>MLSEGTHLRPYETLGAHADTMDGVTGTRFSVWAPNARRVSVVGQFNYWDGRRHPMRLRKESGIWELFIPGAHNGQLYKYEMIDANGNLRLKSDPYAFEAQMRPETASLICGLPEKVVQTEERKKANQFDAPISIYEVHLGSWRRHTDNNFWLSYRELADQLVPYAKWMGFTHLELLPINEHPFDGSWGYQPTGLYAPTRRFGTRDDFRYFIDAAHAAGLNVILDWVPGHFPTDDFALAEFDGTNLYEHSDPREGYHQDWNTLIYNYGRREVSNFLVGNALYWIERFGIDALRVDAVASMIYRDYSRKEGEWIPNEFGGRENLEAIEFLRNTNRILGEQVSGAVTMAEESTDFPGVSRPQDMGGLGFWYKWNLGWMHDTLDYMKLDPVYRQYHHDKLTFGILYNYTENFVLPLSHDEVVHGKKSI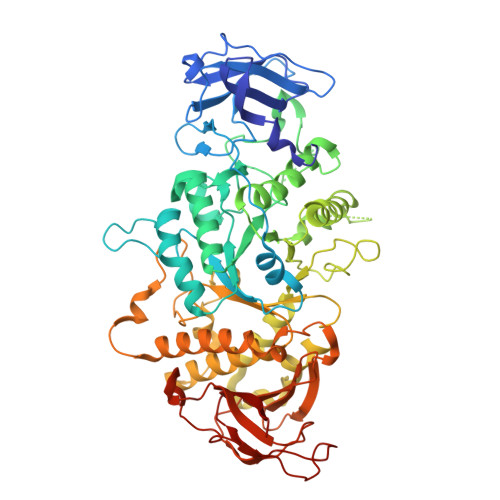LDRMPGDAWQKFANLRAYYGWMWAFPGKKLLFMGNEFAQGREWNHDASLDWHLLEGGDNWHHGVQRLVRDLNLTYRHHKAMHELDFDPYGFEWLVVDDKERSVLIFVRRDKEGNEIIVASNFTPVPRHDYRFGINQPGKWREILNTDSMHYHGSNAGNGGTVHSDEIASHGRQHSLSLTLPPLATIWLVREAE[4x]2'-FLUORO-2'-DEOXYURIDINE 3'-MONOPHOSPHATE | C9 H12 F N2 O8 P | 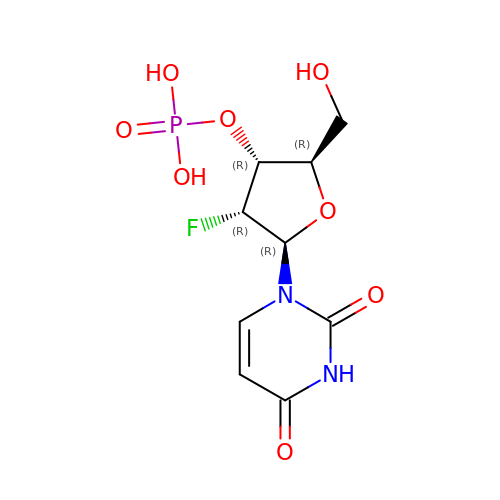IFIXUMAFUNKIAA-XVFCMESISA-N> EETLMDSTTATAELGWMVHPPSGWEEVSGYDENMNTIRTYQVCNVFESSQNNWLRTKFIRRRGAHRIHVEMKFSVRDCSSIPSVPGSCKETFNLYYYEADFDLATKTFPN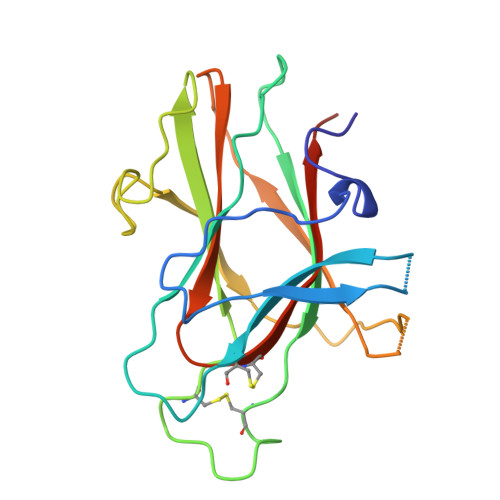WMENPWVKVDTIAADESFSQVDLGGRVMKINTEVRSFGPVSRNGFYLAFQDYGGCMSLIAVRVFYRKCPRIIQ>[3x]EWSHPQFEKGGIAKIDVHNIEDIEQYKKAITQKLQTSLSLFKYAKTKNLPHIKPIYKYITIEGTETAEGIESAYIESEVPALAGTSIGFKINSKEGKHLLDVIAYVKSASYSSVYTKLYSTGPTSGINTKHDELCTGPCPANINHQVGWLTFARERTSSHGCEEFGCLAVSD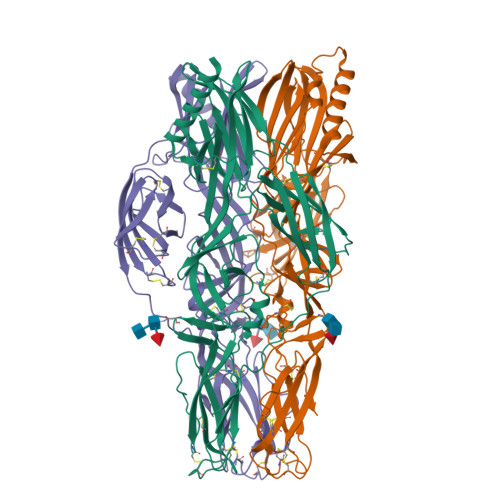GCVFGSCQDIIKEELSVYRKETEEVTDVELCLTFSDKTYCTNLNPVTPIITDLFEVQFKTVETYSLPRIVAVQNHEIKIGQINDLGVYSKGCGNVQKVNGTIYGNGVPRFDYLCHLASRKEVIVRKCFDNDYQACKFLQSPASYRLEEDSGTVTIIDYKKILGTIKMKAILGDVKYKTFADSVDITAEGSCTGCINCFENIHCELTLHTTIEASCPIKSSCTVFHDRILVTPNEHKYALKMVCTEKPGNTLTIKVCNTKVEASMALVDAKPIIELAPVDQTAYIRE> GHMKKVKSLFLLVLGNTEISTIPGISVAGATPELTKI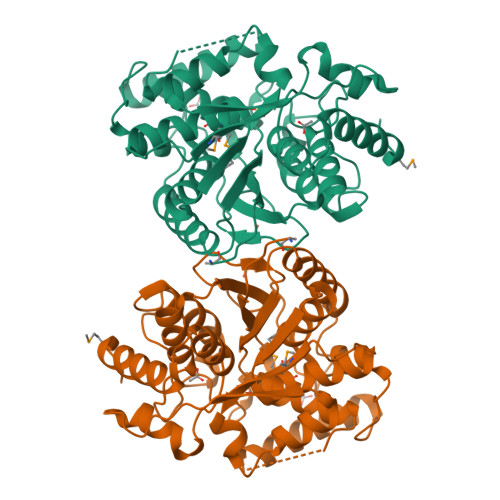TPVADAEYLFYEKPLTIDTIPVTPEGHPTPAIITKAARELSNFPILVVRGGTYLAPLIPHVHISNVVGRDFRREPALPEVEVIIERAKLLGKELEKIANEIVIGESTPGGTTTAQAILWALGYEAKTSSASPENPQELKEKVIKEGFKRVGIEKGGLKDKPLEALKEFGDPMIATVLGLSLGFGGDVVLAGGTQMLAVSALLKSLGEDLSRFMIATTRWVVEDPSATFIETAREIGIISYVAELDFSKSKFKGLRDYERGYVKEGVGAGGATWLAVKAGYSPEDVSKKVEELYERLMGLR N-benzyl-2-(2,6-dimethylanilino)-N,N-diethyl-2-oxoethan-1-aminium | C21 H29 N2 O | 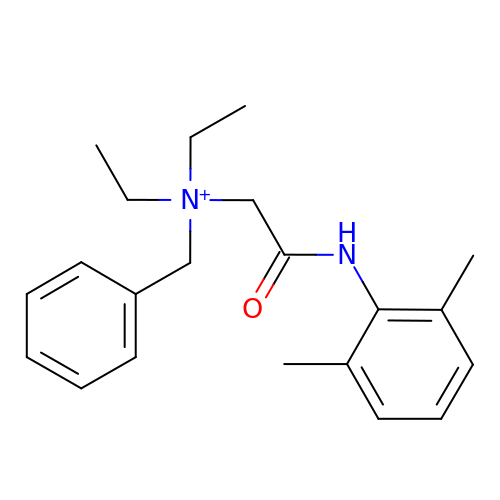ZFQMTVNLDNXRNQ-UHFFFAOYSA-O>[2x]MSLVLNDLLICCRQLEHDRATERKKEVEKFKRLIRDPETIKHLDRHSDSKQGKYLNWDAVFRFLQKYIQKETECLRIAKPNVSASTQASRQKKMQEISSLVKYFIKCANRRAPRLKCQELLNYIMDTVKDSSNGAIYGADCSNILLKDILSVRKYWCEISQQQWLELFSVYFRLYLKPSQDVHRVLVARIIHAVTKGCCSQTDGLNSKFLDFFSKAIQCARQEKSSSGLNHILAALTIFLKTLAVNFRIRVCELGDEILPTLLYIWTQHRLNDSLKEVIIELFQLQIYIHHPKGAKTQEKGAYESTKWRSILYNLYDLLVNEISHIGSRGKYSSGFRNIAVKENLIELMADICHQVFNEDTRSLEISQSYTTTQRESSDYSVPCKRKKIELGWEVIKDHLQKSQNDFDLVPWLQIATQLISKYPASLPNCELSPLLMILSQLLPQQRHGERTPYVLRCLTEVALCQDKRSNLESSQKSDLLKLWNKIWCITFRGISSEQIQAENFGLLGAIIQGSLVEVDREFWKLFTGSACRPSCPAVCCLTLALTTSIVPGTVKMGIEQNMCEVNRSFSLKESIMKWLLFYQLEGDLENSTEVPPILHSNFPHLVLEKILVSLTMKNCKAAMNFFQSVPECEHHQKDKEELSFSEVEELFLQTTFDKMDFLTIVRECGIEKHQSSIGFSVHQNLKESLDRCLLGLSEQLLNNYSSEITNSETLVRCSRLLVGVLGCYCYMGVIAEEEAYKSELFQKAKSLMQCAGESITLFKNKTNEEFRIGSLRNMMQLCTRCLSNCTKKSPNKIASGFFLRLLTSKLMNDIADICKSLASFIKKPFDRGEVESMEDDTNGNLMEVEDQSSMNLFNDYPDSSVSDANEPGESQSTIGAINPLAEEYLSKQDLLFLDMLKFLCLCVTTAQTNTVSFRAADIRRKLLMLIDSSTLEPTKSLHLHMYLMLLKELPGEEYPLPMEDVLELLKPLSNVCSLYRRDQDVCKTILNHVLHVVKNLGQSNMDSENTRDAQGQFLTVIGAFWHLTKERKYIFSVRMALVNCLKTLLEADPYSKWAILNVMGKDFPVNEVFTQFLADNHHQVRMLAAESINRLFQDTKGDSSRLLKALPLKLQQTAFENAYLKAQEGMREMSHSAENPETLDEIYNRKSVLLTLIAVVLSCSPICEKQALFALCKSVKENGLEPHLVKKVLEKVSETFGYRRLEDFMASHLDYLVLEWLNLQDTEYNLSSFPFILLNYTNIEDFYRSCYKVLIPHLVIRSHFDEVKSIANQIQEDWKSLLTDCFPKILVNILPYFAYEGTRDSGMAQQRETATKVYDMLKSENLLGKQIDHLFISNLPEIVVELLMTLHEPANSSASQSTDLCDFSGDLDPAPNPPHFPSHVIKATFAYISNCHKTKLKSILEILSKSPDSYQKILLAICEQAAETNNVYKKHRILKIYHLFVSLLLKDIKSGLGGAWAFVLRDVIYTLIHYINQRPSCIMDVSLRSFSLCCDLLSQVCQTAVTYCKDALENHLHVIVGTLIPLVYEQVEVQKQVLDLLKYLVIDNKDNENLYITIKLLDPFPDHVVFKDLRITQQKIKYSRGPFSLLEEINHFLSVSVYDALPLTRLEGLKDLRRQLELHKDQMVDIMRASQDNPQDGIMVKLVVNLLQLSKMAINHTGEKEVLEAVGSCLGEVGPIDFSTIAIQHSKDASYTKALKLFEDKELQWTFIMLTYLNNTLVEDCVKVRSAAVTCLKNILATKTGHSFWEIYKMTTDPMLAYLQPFRTSRKKFLEVPRFDKENPFEGLDDINLWIPLSENHDIWIKTLTCAFLDSGGTKCEILQLLKPMCEVKTDFCQTVLPYLIHDILLQDTNESWRNLLSTHVQGFFTSCLRHFSQTSRSTTPANLDSESEHFFRCCLDKKSQRTMLAVVDYMRRQKRPSSGTIFNDAFWLDLNYLEVAKVAQSCAAHFTALLYAEIYADKKSMDDQEKRSLAFEEGSQSTTISSLSEKSKEETGISLQDLLLEIYRSIGEPDSLYGCGGGKMLQPITRLRTYEHEAMWGKALVTYDLETAIPSSTRQAGIIQALQNLGLCHILSVYLKGLDYENKDWCPELEELHYQAAWRNMQWDHCTSVSKEVEGTSYHESLYNALQSLRDREFSTFYESLKYARVKEVEEMCKRSLESVYSLYPTLSRLQAIGELESIGELFSRSVTHRQLSEVYIKWQKHSQLLKDSDFSFQEPIMALRTVILEILMEKEMDNSQRECIKDILTKHLVELSILARTFKNTQLPERAIFQIKQYNSVSCGVSEWQLEEAQVFWAKKEQSLALSILKQMIKKLDASCAANNPSLKLTYTECLRVCGNWLAETCLENPAVIMQTYLEKAVEVAGNYDGESSDELRNGKMKAFLSLARFSDTQYQRIENYMKSSEFENKQALLKRAKEEVGLLREHKIQTNRYTVKVQRELELDELALRALKEDRKRFLCKAVENYINCLLSGEEHDMWVFRLCSLWLENSGVSEVNGMMKRDGMKIPTYKFLPLMYQLAARMGTKMMGGLGFHEVLNNLISRISMDHPHHTLFIILALANANRDEFLTKPEVARRSRITKNVPKQSSQLDEDRTEAANRIICTIRSRRPQMVRSVEALCDAYIILANLDATQWKTQRKGINIPADQPITKLKNLEDVVVPTMEIKVDHTGEYGNLVTIQSFKAEFRLAGGVNLPKIIDCVGSDGKERRQLVKGRDDLRQDAVMQQVFQMCNTLLQRNTETRKRKLTICTYKVVPLSQRSGVLEWCTGTVPIGEFLVNNEDGAHKRYRPNDFSAFQCQKKMMEVQKKSFEEKYEVFMDVCQNFQPVFRYFCMEKFLDPAIWFEKRLAYTRSVATSSIVGYILGLGDRHVQNILINEQSAELVHIDLGVAFEQGKILPTPETVPFRLTRDIVDGMGITGVEGVFRRCCEKTMEVMRNSQETLLTIVEVLLYDPLFDWTMNPLKALYLQQRPEDETELHPTLNADDQECKRNLSDIDQSFNKVAERVLMRLQEKLKGVEEGTVLSVGGQVNLLIQQAIDPKNLSRLFPGWKAWV

Ataxia-telangiectasia mutated (ATM) is a large protein kinase with a central role in the cellular response to DNA double-strand breaks (DSBs) and related genotoxic stress. ATM, which belongs to the phosphatidylinositol 3-kinase-like protein kinase (PIKK) family, is essential for the sensing of DSBs during the cell cycle. MRN contributes to the localization of ATM to DSBs, and together with double-stranded DNA (dsDNA), it activates ATM as a protein kinase.

Cryo-EM samples were prepared by mixing ATM with the non-hydrolyzable ATP analog adenylyl-imidodiphosphate (AMP-PNP) and MgCl2. The cryo-EM data yielded a consensus reconstruction in point group C2 that extended to an overall resolution of 2.5 Å as determined from gold standard Fourier shell correlation (FSC = 0.143). The refined model contains over 90% of the ATM residues, with the remaining residues in poorly-ordered or disordered loops. The ATM FAT domain plays a central role in dimerization, which buries ~3800 Å2 of surface area on each ATM protomer (Krissinel and Henrick, 2007). (Baretić et al., 2017; Xin et al., 2019; Jansma et al., 2020; Yates et al., 2020), the kα9b helix occludes part of the putative substrate-binding site, and the packing of the coiled coil against it may well stabilize this autoinhibitory conformation. The adenine ring is sandwiched between hydrophobic or aromatic residues from the N lobe (Leu2715, Leu2767, and Trp2769) and C lobe (Leu2877 and Ile2889), whereas the N6 and N1 groups hydrogen bond to backbone carbonyl and amide groups of Glu2768 and Cys2770, respectively. The Mg2+ ion, which contacts the AMP-PNP α phosphate group, is coordinated by Asn2875 and Asp2889 of the C lobe – interactions conserved among both PIKKs and canonical protein kinases. In this superposition, the ATM N lobe is positioned remarkably similar to those of inactive mTOR and inactive DNA-PKcs, with the three N lobes forming a tightly clustered set clearly distinct from the cluster of active mTOR and active DNA-PKcs N lobes. The positions of the N lobe hairpin and other ATP-interacting residues relative to the C lobe catalytic and magnesium-coordinating residues are much closer to those of the inactive mTOR and DNA-PKcs structures compared the active ones. This positioning thus suggests that in addition to relieving the blockage of the substrate-binding site, the activation of ATM may well involve a conformational change within the FAT domain and the associated change in the relative orientation of the N and C lobes of the kinase domain. Our cryo-EM structure of human ATM shows an overall symmetric dimer, albeit with the Pincer and Spiral domains exhibiting some mobility arising from conformational flexibility within the Pincer domain.> GVPTYLLPGSSQFMTTDDHSSAPAFPDFSPTPEIHIPGRVHNMLELVQVESMMEINNV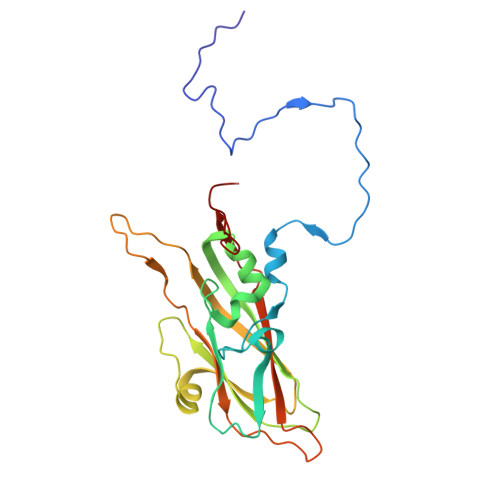AGSSGMERLRVEISVQTDMDALLFNIPLDIQLDGPLRSTLLANIARYYTHWSGSMEMTFMFCGSFMATGKVILCYTPPGGSCPTDRESAMLGTHIVWDFGLQSSITLVIPWISGSHFRMFNSDAKSINANVGYVTCFMQTNLIVPKEAATSTYIIGFAAAKNDFSLRLMRDSPDIGQSQQLE Central to the stringent response are the two unusual nucleotides ppGpp and pppGpp (collectively (p)ppGpp or alarmones). In contrast, short RSH-type alarmone synthetases only contain a synthetase domain and lack the hydrolase domain as well as regulatory domains found within the CTD of long RSH proteins. Members of this ‘small alarmone synthetase’ (SAS) family fall into the RelQ (also: SAS1) and RelP (also: SAS2) subclasses and are found in a wide range of bacteria including Bacillus subtilis, Staphylococcus aureus, Enterococcus faecalis and Listeria monocytogenes. In summary, RelP always appears as a highly active alarmone synthetase, while RelQ can switch between a passive state with low and an active (i.e. pppGpp-stimulated) state with high (p)ppGpp synthetase activity.

To gain further insights into the disparate enzymatic activities of RelQ and RelP, we attempted to solve the structure of SaRelP in presence of the non-hydrolysable ATP analogue AMPCPP (α,β-methyleneadenosine 5′-triphosphate) and GDP or GTP. However, we could only obtain crystals and solve the structure of SaRelP in presence of AMPCPP. Coordination of AMPCPP within all the four active sites of SaRelP is guided by π-stacking interactions of the adenine base with the arginine residues 78 and 112 of SaRelP. The ribose moiety of the adenosine is coordinated by hydrogen bonding via His190. Interactions with the phosphate moieties of AMPCPP are mainly established by lysine and arginine residues residing in β1 and α2 (i.e. Lys80, Lys88 and Arg91) and Ser84 contacting the 5′ α-phosphate. AMPCPP adopts a kinked conformation that is enforced by a magnesium ion coordinated by Asp107 and Glu174. As all ATP-coordinating and catalytic amino acid residues are strictly conserved among RelP/RelQ proteins, we suspect a common ATP-binding mode and mode of catalysis. In stark contrast, the G-Loop of SaRelP was well-ordered and could be unambiguously modeled in its apo- and ATP-bound structures. Our analysis demonstrates that binding of ATP proceeds in identical fashion in RelP/RelQ proteins, because both proteins harbor an identical architecture of their ATP-coordination site.

>[2x]MGHHHHHHYVDRKPSLYLEDLRHDFKNSLSKFENGDEAFDTLLGFVELDHIYSSALKEISTKLSILDDNFNHIYKHNPIHHMERRVKEMRSLIEKLNRKGLQISAETAKEHILDIAGIRVVCNYLDDIYLIEEMLLKQEDVQLIKRKDYIQHPKENGYRSLHIVVSIPVFLAERVEVLPVEIQIRTIGMDMWASLEHKIRYKNNAETEKYRDLLKECATEITEVEDKLQQIHSEITE Flavin-containing monooxygenases (FMOs, EC 1.14.13.8) are enzymes that insert one molecule of oxygen into organic substrates using the cofactors flavin adenine dinucleotide (FAD) and NAD(P)H (1–3). A subgroup of bacterial FMOs oxidize trimethylamine (TMA) to trimethylamine N-oxide (TMAO) and are often referred to as trimethylamine monooxygenases (Tmms). The mFMO enzyme forms a dimer, and each monomer consists of two domains: the larger FAD-binding domain and the smaller NADPH-binding domain. Upon binding, NADPH reduces the tightly bound FAD, thus generating the reactive flavin intermediate C4a-hydroperoxy-FAD and NADP+.

To make the flavin-containing monooxygenase (FMO) Methylophaga aminisulfidivorans trimethylamine monooxygenase (mFMO) more suitable for industrial application, we engineered it using the Protein Repair One-Stop Shop (PROSS) algorithm. The melting temperature (Tm) of native mFMO was measured to be 46.2°C, which is in line with the previously reported Tm of 46.7°C. All mFMO variants demonstrated increased temperature stability compared to that of the wild-type enzyme, as reflected by their Tm values, which ranged from 50.9°C for mFMO_28 to 55.2°C for mFMO_20. To understand the structural basis for the increased thermostability of mFMO_20, we crystallized it with the cofactors FAD and NADPH. The crystals were indexed in the C2221 space group and contained the biological dimer within the asymmetric unit, with one FAD and one NADP+ molecule bound per catalytic site. Interestingly, half of the mFMO_20 mutations are located in a 46-amino-acid subsequence (M353Q to L398K) of a region in the large domain containing three helices: α6 (K345 to T361), α7 (A365D to M382), and α8 (I390 to N406). Structural analysis revealed that five of these mutated residues form new salt bridges involving six native residues (K358R-D374, L360E-R356, A365D-K401, N378D-K300-D351, and L398K-E366), four of which form interhelical interactions, thus confirming the PROSS model predictions. Helices α6 and α7 are directly connected by K358R-D374 and indirectly connected, via the β18-β19 loop, by N378D-K300-D351. Helices α7 and α8 are connected by A365D-K401 and L398K-E366. Two new hydrogen bonds involving side chains are also introduced, one forming an intrahelical bond (α6; M353Q-R356) and the other an interhelical bond (α7-α8; T370D-N394). The lower B-factors observed near the entrance to the active site in our crystallographic analysis are consistent with the increased thermal and kinetic stability of this design.

>[2x]MATRIAILGAGPSGMAQLRAFQSAQEKGAEIPELVCFEKQADWGGQWNYTWRTGLDENGEPVHSSMYRYLWSNGPKECLEFADYTFDEHFGKPIPSYPPREVLWDYIKGRVEKAGVRKYIRFNTAVRHVEFNEDTQTFTVTVQDHTTDTIYSEEFDYVVCCTGHFSTPYVPEFEGFEKFGGRILHAHDFRDALEFKGKTVLLVGSSYSAEDIGSQCYKYGAKKVISCYRTAPMGYDWPENWDERPNLVRVDGENAYFADGSSEKVDAIILCTGYIHHFPFLNDDLRLVTDNRLWPPNLYKGVVWEDNPKFFYIGMQDQWYSFNMFDAQAWYARDVIMGRIPLPSKEEMKADSQAWREREETLKTDEEMYDFQGDYIQDLIDMTDYPSFDIPAVNKTFKEWKHHKKENIMTFRDHSYRSLMTGTMAPKHHTPWIDALDDSLEAFLSDKSEIPVAKEALEHHHHHH> MKDLVDTTEMYLRTIYELEAEGVTPLRARIAERLEQ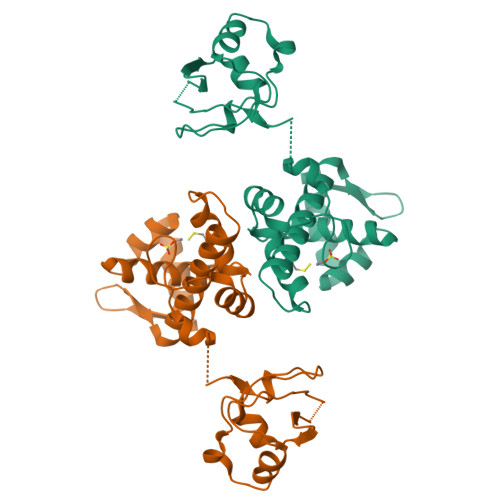SGPTVSQTVARMERDGLVVVASDRSLQMTPTGRTLATAVMRKHRLAERLLTDIIGLDINKVHDEACRWEHVMSDEVERRLVKVLKDVSRSPFGNPIPGLDELGVGNSDAAAPGTRVIDAATSMPRKVRIVQINEIFQVETDQFTQLLDADIRVGSEVEIVDRDGHITLSHNGKDVELLDDLAHTIRIEEL>[2x]MGSGSSSYRPKAIYLDIDGRIQKVIFSKYCNSSDIMDLFCIATGLPRNTTISLLTTDDAMVSIDPTMPANSERTPYKVRPVAIKQLSEREELIQSVLAQVAEQFSRAFKINELKAEVANHLAVLEKRVELEGLKVVEIEKCKSDIKKMREELAARSSRTNCPCKYSFLDNHKKLTPRRDVPTYPKYLLSPETIEALRKPTFDVWLWEPNEMLSCLEHMYHDLGLVRDFSINPVTLRRWLFCVHDNYRNNPFHNFRHCFCVAQMMYSMVWLCSLQEKFSQTDILILMTAAICHDLDHPGYNNTYQINARTELAVRYNDISPLENHHCAVAFQILAEPECNIFSNIPPDGFKQIRQGMITLILATDMARH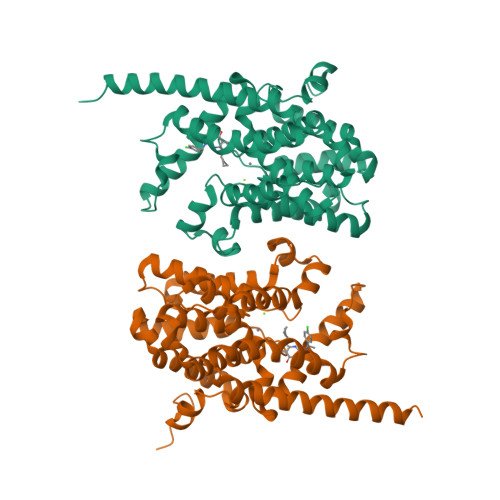AEIMDSFKEKMENFDYSNEEHMTLLKMILIKCCDISNEVRPMEVAEPWVDCLLEEYFMQSDREKSEGLPVAPFMDRDKVTKATAQIGFIKFVLIPMFETVTKLFPMVEEIMLQPLWESRDRYEELKRIDDAMKELQKKTDSLTSGATEKSRERSRDVKNSEGDCA>MGETIAIVGGTLIDGNGGVPVPETTVFIEDGRITKVGSTDQIEVHPNIRQIDAQGKWILPGLVNGNVHLLDGIMMMGRGGIEYLARFEGNYYKVIEEAAQIALRGGVTTVFDTWNALEPVTIARDRIASGAAEGARIFFAGTLIGMGGPFTGDFMRPSMQARTVMSRTFADRMDAMFEVGMGRHLSTLPPAEVRPLIREYLERGVDFCKIAVTDHLVGLLGFRAPYFTFSERVLDVLVDEVRRAGVPLLTHTTSLEGLNTAIERDADLMIHATMTGQAPIP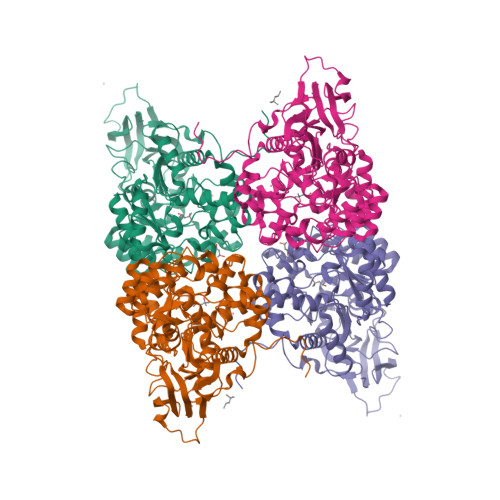EETIEKLLEKQLWSEVQPTTIAQQAWMDSVDHPFADFSGRVHHENDVRMIKAGVPLVLGTDAGCTDPDILEDMSQGELHERPWTLGEDHFVWMQAMVEKGMDPMAAILAGTANPAKAYRKFDELGSIDVGKLGDVVVLDQDPLADITNMRTLSHVVKEGREIDFHGLPLSPLVTAYPRTANVLD[4x]>[6x]GSHMASMTGGQQMGRGSMSKIVKIIGREIIDSRGNPTVEAEVHLEGGFVGMAAAPSGASTGSREALELRDGDKSRFLGKGVTKAVAAVNGPIAQALIGKDAKDQAGIDKIMIDLDGTENKSKFGANAILAVSLANAKAAAAAKGMPLYEHIAELNGTPGKYSMPVPMMNIINGGEHADNNVDIQEFMIQPVGAKTVKEAIRMGSEVFHHLAKVLKAKGMNTAVGDEGGYAPNLGSNAEALAVIAEAVKAAGYELGKDITLAMDCAASEFYKDGKYVLAGEGNKAFTSEEFTHFLEELTKQYPIVSIEDGLDESDWDGFAYQTKVLGDKIQLVGDDLFVTNTKILKEGIEKGIANSILIKFNQIGSLTETLAAIKMAKDAGYTAVISHRSGETEDATIADLAVGTAAGQIKTGSMSRSDRVAKYNQLIRIEEALGEKAPYNGRKEIKGQA

Bacterial enolase, a metalloenzyme involved in carbon metabolism, is essential to bacterial glycolysis and the generation of metabolites used in several bacterial cell processes. Enolase, a multifunctional metalloenzyme, catalyzes the dehydration of 2-phosphoglycerate (2-PGA) to phosphoenolpyruvate (PEP) through the intermediacy of a stabilized carbanion. Prokaryotes express a single isoform of enolase which, in addition to acting as a key mediator of energy production, appears to be involved in the overall infection process - enhancing bacterial resistance, invasiveness, and tissue damage. Herein, we present novel crystal structures of E. coli enolase in complex with SF2312 and its oxidized derivative, KSF where the C5 hemiaminal is oxidized to an imide carbonyl unit.

While there is full density for SF2312 ligand in all six monomers, KSF is present in only three out of the six active sites. Interestingly, in the ligand unbound sites we instead observed density for tartrate, which is a component of the crystallization medium. Unlike in the E. coli enolase:SF2312 structure, Loop 2 (residues 154–165) and Loop 3 (residues 248–268) are disordered and Mg2 is absent from the active site of the enolase:KSF complex. The three monomers containing KSF all adopt the same conformation with an average RMSD of 0.29, however in chain E, the pyrrolidine is flipped ~135° compared to chains D and F where KSF adopts a similar orientation to SF2312. Similar to SF2312, the bidentate hydroxamate of KSF completes the octahedral coordination of Mg1 while hydrogen bonding with the charged side chains of Gln166, Asp316, and Lys392. The phosphonate group of KSF is also within hydrogen bonding distance of Arg370, Ser371, Ser41, and Lys341. Importantly, the change in hybridization of C5 from sp3 tetrahedral geometry in SF2312 to sp2 trigonal planar geometry in KSF more accurately reflects the geometry of the PEP product rather than the anionic intermediate. The downstream effect of this observation manifests in a very significant reorientation of the phosphate group which no longer interacts with His158 and completely destabilizes Loops 2 and 3. This major conformational change is reflected in over 400-fold loss in activity between SF2312 and KSF (SF2312 IC50: 18.4 ± 2.84 nM, KSF IC50: 7.67 ± 0.38 µM).> TESVISGSPAWGLDGILELKEYLWFAAKQTDSYRTYQIERGHPDVKVALIDSGLDLDHPDLKASVNTNGGWNYIDGKPVSGDPTGHGTQTAGMINIIAPDVTITPYQVLDEKGGDSYNIMKAMVDAVNDGHEVINISTGSYTSLDREGKVLMKAYQRAANYAAKHQVLVFSSAGNKGVNLDEMRKTENKVHLPSALKHVVSVGSNMKSNNISPYSNQGREIEFTAPGGYLGETYDQDGMVRVTDLVLTTYPKGKDNTALDQMLNIPKGYSLSYGTSLAAPQVAGTAALVISEYRER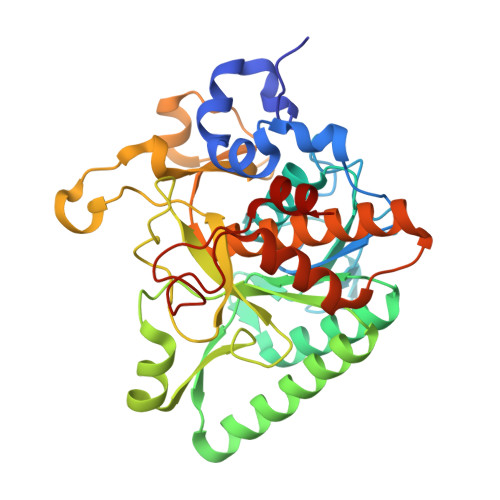HHRKPSAKQVHHILRKSALDLGKPGKDVIYGYGEVRAYQALKMMNKE>[24x]MAIEIKVPDIGADEVEITEILVKVGDKVEAEQSLITVEGDKASMEVPSPQAGIVKEIKVSVGDKTQTGALIMIFDSADGAADAAPAQAEEKKEAAPAAAPAAAAAKDVNVPDIGSDEVEVTEILVKVGDKVEAEQSLITVEGDKASMEVPAPFAGTVKEIKVNVGDKVSTGSLIMVFEVAGEAGAAAPAAKQEAAPAAAPAPAAGVKEVNVPDIGGDEVEVTEVMVKVGDKVAAEQSLITVEGDKASMEVPAPFAGVVKELKVNVGDKVKTGSLIMIFEVEGAAPAAAPAKQEAAAPAPAAKAEAPAAAPAAKAEGKSEFAENDAYVHATPLIRRLAREFGVNLAKVKGTGRKGRILREDVQAYVKEAIKRAEAAPAAT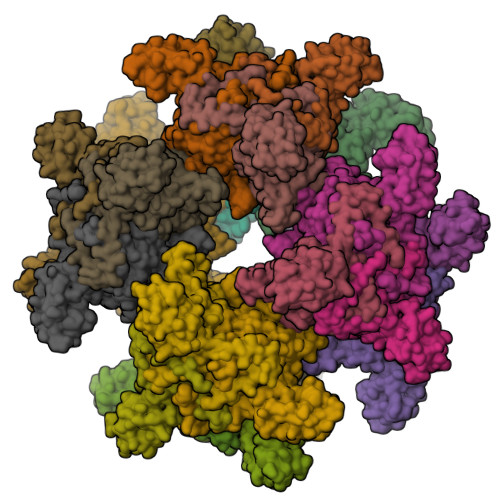GGGIPGMLPWPKVDFSKFGEIEEVELGRIQKISGANLSRNWVMIPHVTHFDKTDITELEAFRKQQNEEAAKRKLDVKITPVVFIMKAVAAALEQMPRFNSSLSEDGQRLTLKKYINIGVAVDTPNGLVVPVFKDVNKKGIIELSRELMTISKKARDGKLTAGEMQGGCFTISSIGGLGTTHFAPIVNAPEVAILGVSKSAMEPVWNGKEFVPRLMLPISLSFDHRVIDGADGARFITIINNTLSDIRRLVM>LQERDIVPVDASYEVKELYVPENKLHLAKTDAETLPALKINKVDMQWVQVLAEGWATPLNGFMREREYLQCLHFDCLLDGGVINLSVPIVLTATHEDKERLDGCTAFALMYEGRRVAILRNPEFFEHRKEERCARQWGTTCKNHPYIKMVMEQGDWLIGGDLQVLDRVYWNDGLDQYRLTPTELKQKFKDMNADAVFAFQLRNPVHNGHALLMQDTHKQLLERGYRRPVLLLHPLGGWTKDDDV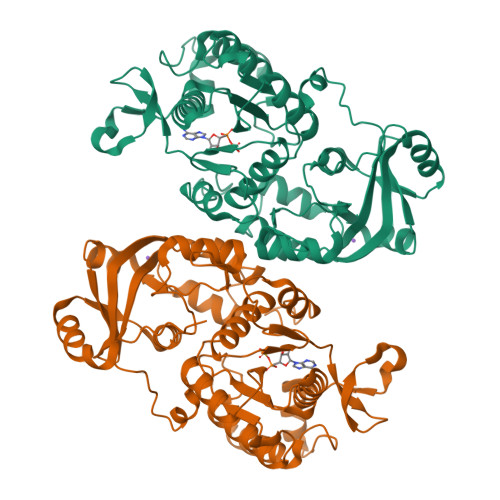PLMWRMKQHAAVLEEGVLNPETTVVAIFPSPMMYAGPTEVQWHCRARMVAGANFYIVGRDPAGMPHPETGKDLYEPSHGAKVLTMAPGLITLEIVPFRVAAYNKKKKRMDYYDSEHHEDFEFISGTRMRKLAREGQKPPEGFMAPKAWTVLTEYYKSLEKA[2x]>MSHGKQFTLYTHKGGPNGWKVTIVLEELGLTYESIFLDFQKGEHKAPEYLKVNPNGRIPALIDHKNNDYTVWESNAIIQYLVDKYDKDRKVSVAPGTNEYYTQLQWLYFQASGQGPYYGQAAWFSVYHPEKVPSAIERYRNEIKRVLGVLESVLSKQEFLVDGKATVADFSFLPWNEGAAKFLLEGSQFEEEFPATA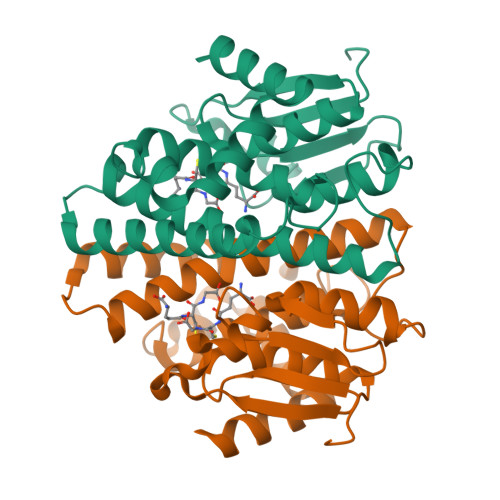KWHKKLLERPAIAKVWEERAKVSAH[2x]>MRINHNIAALNTLNRLSSNNSASQKNMEKLSSGLRINRAGDDAAGLAISEKMRGQIRGLEMASKNSQDGISLIQTAEGALTETHAILQRVRELVVQAGNTGTQDKATDLQSIQDGISALTDEIDGISNRTEFNGKKLLDGTYKVDTATPANQKNLVFQIGANATQQISVNIEDMGADALGIKEADGSIAALHSVNDLDVTKFADNAADCADIGFDAQLKVVDEAINQVSSQRAKLGAVQNRLEHTINNLSASGENLTAAESRIRDVDMAKEMSEFTKNNILSQA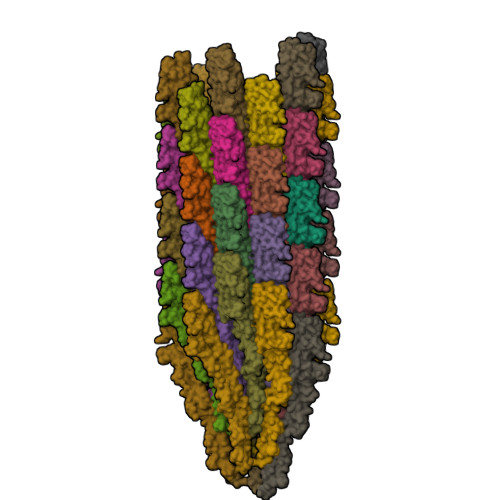SQAMLAQANQQPQNVLQLLR[46x]> MGEYFVKFLKEKYPDAKEIPYAELLGILSAQPTWDRSNGFHSVVDQYPEFKMVAQQSAEFDRDTAYKVTEQILQAHPEIKAIWCGNDAMALGAMKACEAAGRTDIYIFGFDGAEDVINAIKEGKQIVATIMQFPKLMARLAVEWADQYLRGERSFPEIVPVTVELVTRENIDKYT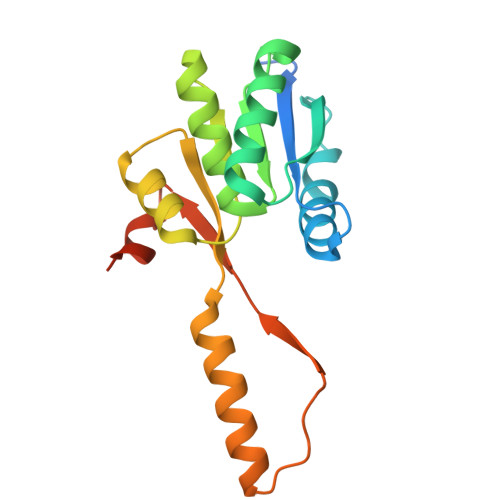AYGRKLEHHHHHH>[6x]GEDSLTKQPEEVFDVLEKLGEGSYGSVFKAIHKESGQVVAIKQVPVESDLQEIIKEISIMQQCDSPYVVKYYGSYFKNTDLWIVMEYCGAGSVSDIIRLRNKTLIEDEIATILKSTLKGLEYLHFMRKIHRNIKAGNILLNTE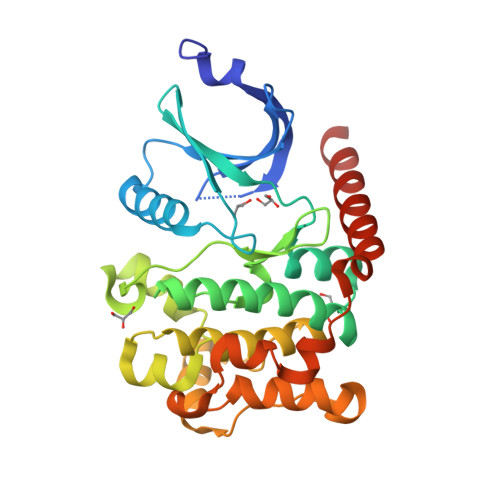GHAKLADFGVAGQLTDTMAKRNTVIGTPFWMAPEVIQEIGYNCVADIWSLGITSIEMAEGKPPYADIHPMRAIFMIPTNPPPTFRKPELWSDDFTDFVKKCLVKNPEQRATATQLLQHPFIKNAKPVSILRDLITEAMEIKAKRHEEQQRELEEEE>SEFKETPELESAVRAMEAAA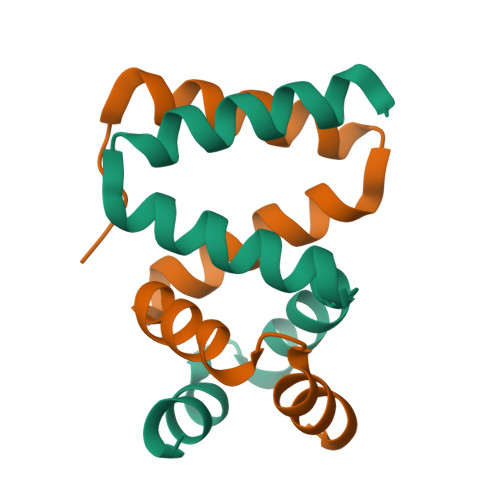NVDPLFQSALSVFMWLEENGIVTDMANFALSDPNAHRMRNFLANA[2x]> GPLGSASLQRRSDFCGQWDTATAGDFTLYNDLWGESAGTGSQCTGVDSYSGDTIAWHTSWSWSGGSSSVKSYVNAALTFTPTQLNCISSIPTTWKWSYSGSSIVADVAYDTFLAETASGSSKYEIMVWLAALGGAGPISSTGSTIATPTIAGVNWKLYSGPNGDT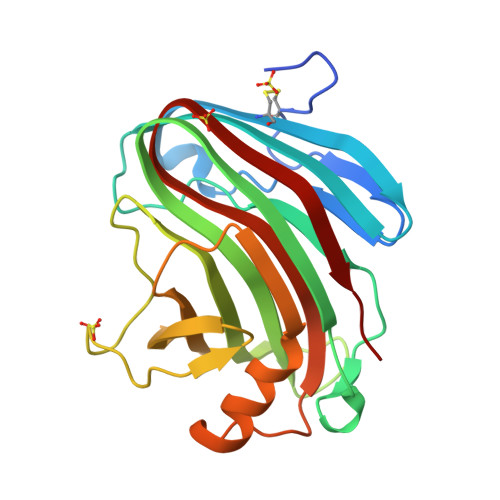TVYSFVADSTTESFSGDLNDFFTYLVDNEGVSDELYLTTLEAGTEPFTGSNAKLTVSEYSISIE>[2x]MALVPVGMAPRQMRVNRCIFASIVSFDACITYKSPC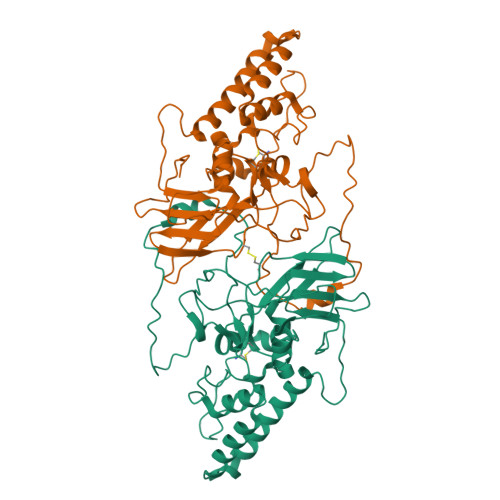SPDAYHDDGWFICNNHLIKRFKMSKMVLPIFDEDDNQFKMTIARHLVGNKERGIKRILIPSATNYQDVFNLNSMMQAEQLIFHLIYNNENAVNTICDNLKYTEGFTSNTQRVIHSVYATTKSILDTTNPNTFCSRVSRDELRFFDVTNARALRGGAGDQLFNNYSGFLQNLIRRAVAPEYLQIDTEELRFRNCATCIIDETGLVASVPDGPELYNPIRSSDIMRSQPNRLQIRNVLKFEGDTRELDRTLSGYEEYPTYVPLFLGYQIINSENNFLRNDFIPRANPNATLGGGAVAGPAPGVAGEAGGGIAV[4-(6,7-dimethoxyquinazolin-4-yl)piperidin-1-yl]-[4-(trifluoromethyloxy)phenyl]methanone 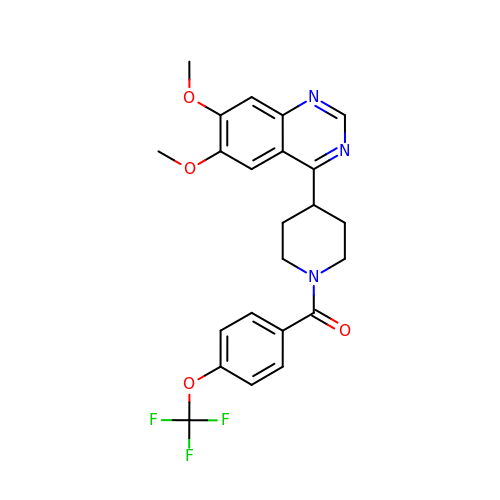| C23 H22 F3 N3 O4 | SRRBAUZQZOASOY-UHFFFAOYSA-N In La Crosse virus, an orthobunyavirus, it has previously been shown that the cap-snatching endonuclease resides in the N-terminal domain of the L protein. The L protein serves as the primary effector, showcasing its multifunctional nature by encompassing both endonuclease (EndoN) activity in its N-terminus and RNA-dependent RNA polymerase (RdRp) activity. During cap-snatching short capped primers derived by endonucleolytic cleavage of host mRNAs by the EndoN are used by the RdRp to initiate the synthesis of vmRNA. The determined atomic structures of different EndoNs show that they harbour a conserved PD…D/ExK catalytic motif in the active site and bind divalent metal ions (Mn2+ or Mg2+) that are critical for catalytic activity.

Crystals of the LACV EndoN–baloxavir complex were obtained following the same procedure as for the L-742,001 complex in the presence of 5 mM MnCl2. The crystal diffracted to 2.2 Å resolution and was processed at 2.64 Å resolution in space group P6122 with four copies of LACV EndoN in the asymmetric unit. The baloxavir structure can be decomposed into two linked tricyclic scaffolds, a metal-chelating scaffold comprising an hydroxypyridotriazinedione motif and a specificity scaffold comprising a dibenzothiepine moiety. One conformation allows the side chain of Asp52 to coordinate the manganese ion Mn2, and the other is in an open form that moves it away from the active site. The chelation of baloxavir, as observed for the chelating DKA motif of L-742,001, occurred via the three coplanar O atoms of the hydroxypyrido­triazinedione motif that bind Mn1 and Mn2; each metal ion displays octahedral coordination with proteic catalytic residues and hydration shell [Fig. 4(c)]. The chelation and specificity motifs of the ligand adopt the same conformations in the active sites of the three molecules. The dibenzothiepine moiety adopts a V shape and makes contact along the Met31 side chain, as for Ile38 in H1N1 FLUAV PA-Nter [Fig. 4(d)]. The chelation and specificity motifs are positioned similarly in the two proteins, despite the absence of the N-terminal end of helix α2 carrying Tyr24 in the LACV EndoN active site, which is responsible for the locking of baloxavir into the H1N1 FLUAV PA-Nter active site. Three molecules of baloxavir were placed (chains A, C and D). The F o − F c density of chain B has a lower quality, making it impossible to locate baloxavir correctly. This is explained by the double conformation of the Tyr49–Phe55 loop containing the catalytic Asp52 residue and the high B factor of Mn2. The R 1 position facing His34 should be substituted by small alkyl groups to reinforce π-stacking interactions, the R 2 position offers the possibility to introduce larger groups and aromatic rings to target inter­actions with Leu30 and Arg33, and in position R 3 there is still more space to extend for buried interactions with Leu30 and Val27.

>GMDYQEYQQFLARINTARDACVAKDIDVDLLMARHDYFGRELCKSLNIEYRNDVPFIDIILDIRPEVDPLTIDAPHITPDNYLYINNVLYIIDYKVSVSNESSVITYDKYYELTRDISDRLSIPIEIVIIRIDPVSRDLHINSDRFKELYPTIVVDINFNQFFDLKQLLYEKFGDDEEFLLKVA[4x]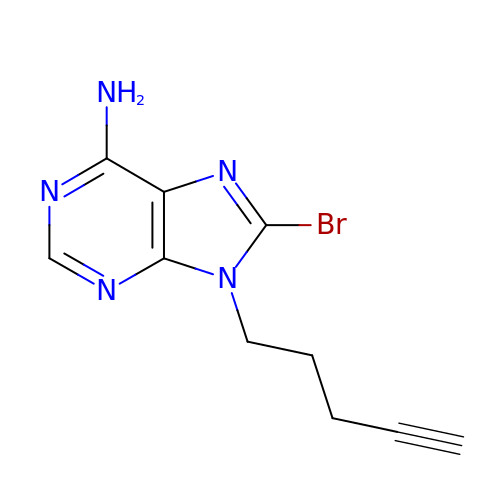8-bromanyl-9-pent-4-ynyl-purin-6-amine | C10 H10 Br N5 | WCMPBWUQKLZDKB-UHFFFAOYSA-N>MSSRSDPGQPMASATDPSGRLALDLTECDREPIHIPGAIQPHGYLFVVSETDLRIASVSANVEDLLRQPPASLLNVPIAHYLTAASAARLTHALHGGDPAAINPIRLDVVTPDGERAFNGILHRHDSIVILELEPRDESRYTNEFFRSVRVAIRRLQTAADLPTACWIAASEVRRITGFDRIKVYQFAADWSGQVIAEDRDSGIPSLLDFHFPSSDIPAQSRALYTINPVRIIPDIGYRPSPLVPDINPRLGGPIDLSFSVLRSVSPTHLEYMVNMGMHAAMSISIVRDNRLWGMISCHNLTPRFVSYEVRQACELIAQVLTWQIGVLEEAEIVRHSVRMRAIQNRLLHELGDEQGLTAGLSRVSEEMLALMGASGFALCSFDGVAAFGRTPSDDEIQALASWLSHRESRGIFQTQQLSASFPEAEVYSDIASGLLAVPLGRASTTLMLWFRPEVAQTVTWGGDPHKPVQIGPRGRRLQTRASFEAWREEVRDRSRPWRSHEIVAAEEIRDLVVD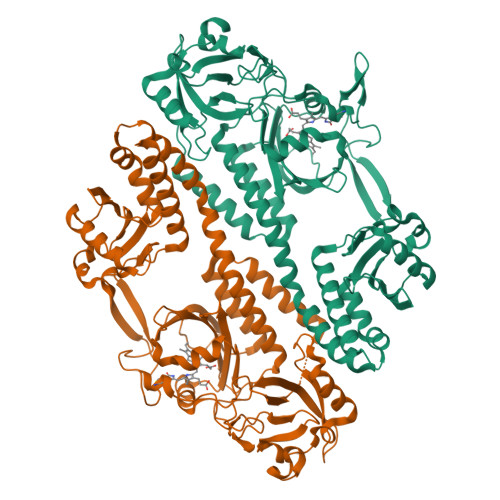VILGRALEHHHHHH[2x]> STSGSGGAIRGIKHIIIVPIPGDSSITTRSRLLDRLVRLIGNPDVSGPKLTGALIGILSLFVESPGQLIQRITDDPDVSIRLLEVVQSDQSQSGLTFASRGTNMEDEADQYFSHDDPISSDQSRFGWFENKEISDIEVQDPEGFNMILGTILAQIWVLLAKAVTAPDTAADSELRRWIKYTQQRRVVGEFRLERKWLDVVRNRIAEDLSLRRFMVALILDIKRTPGNKPRIAEMICDIDTYIVEAGLASFILTIK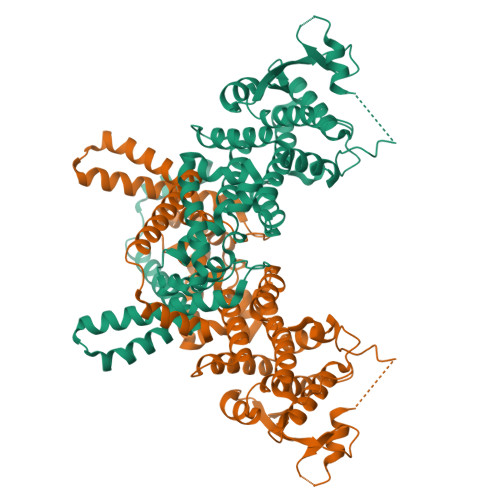FGIETMYPALGLHEFAGELSTLESLMNLYQQMGETAPYMVILENSIQNKFSAGSYPLLWSYAMGVGVELENSMGGLNFGRSYFDPAYFRLGQEMVRRSAGKVSSTLASELGITAEDARLVSEIAMHTTEDKISRMAEEQARHVKNGLECIRALKAEPIGSLAIEEAMAAWSEISDNPGQERA>MRPLKVALVNIPLRVPGSDAWISVPPQGYGGIQWVVANLMDGLLELGHEVFLLGAPGSPAGRPGLTVVPAGEPEEIERWLRTADVDVVHDHSGGVIGPAGLPPGTAFISSHHFTTRPVNPVGCTYSSRAQRAHCGGGDDAPVIPIPVDPARYRSAADQVAKEDFLLFMGRVSPHKGALEAAAFAHACGRRLVLAGP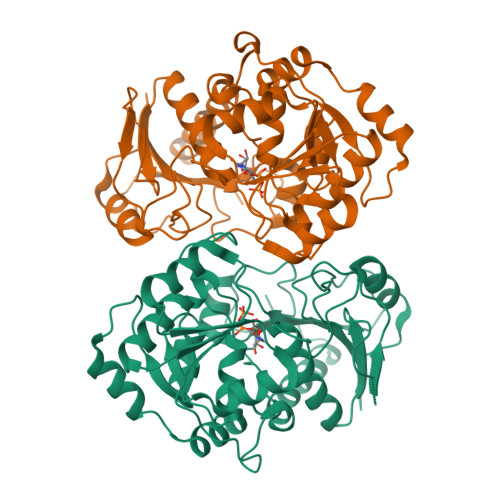AWEPEYFDEITRRYGSTVEPIGEVGGERRLDLLASAHAVLAMSQAVTGPWGGIWCEPGATVVSEAAVSGTPVVGTGNGCLAEIVPSVGEVVGYGTDFAPDEARRTLAGLPASDEVRRAAVRLWGHVTIAERYVEQYRRLLAGATWK[4x]LCAD is a homotetramer containing one FAD per 43 kDa subunit with Glu291 as the catalytic base. LCAD substrate specificity overlaps those of VLCAD and MCAD, and in addition includes unsaturated and branched-chain substrates. Here we present the three-dimensional structure of human LCAD, revealing an unusually large substrate-binding cavity not previously reported in eucaryotic ACADs. The structural basis for the unique substrate binding cavity can be seen in the long E helix, where Pro132 is located in a position to cause unwinding of about two turns of the E helix, thus creating a large cavity.

In addition, the structure of the Glu291Gln (E291Q) mutant complexed with lauric acid has been determined to 2.0 Å resolution. Although we obtained crystals of the LCAD E291Q mutant co-crystallized with substrate lauroyl-CoA (C12-CoA), density for the CoA moiety is not observed, and only weak electron density of the alkyl chain portion is observed, likely due to hydrolysis of C12-CoA during the crystallization process. The crystal packing of the LCAD E291Q P1 form is very similar to the crystal packing of the wild type LCAD P21 crystal, except that, in the P1 space group, the adenine ring binding site now has moved slightly away from the symmetry related A and B molecules to avoid steric clashes, transforming the P21 space group of wild type LCAD to the P1 space group of the E291Q mutant crystal. The chain starts at Glu34 in all four monomers of the mutant LCAD structure. The structure of the catalytic residue mutant, E291Q, with the lauroyl moiety of C12-CoA bound in the active site shows that Gln291, extending out from helix G, is located at the active site close to the Cα-Cβ bond of the substrate. In all eight monomers of E291Q LCAD, electron densities for the substrate fatty-acyl portion are weak and interactions with cavity-forming hydrophobic residues are not seen. The LCAD binding cavity is deeper and wider compared to those of other mammalian ACADs, accounting for the lack of specific interactions between the fatty acyl chain of C12-CoA (bound substrate) and cavity-forming residues. Likewise, the overall structure of ligand-bound E291Q LCAD is similar to those of both the ligand bound and unliganded wild-type structures. In all LCAD structures lacking bound CoA derivatives (all eight monomers of mutant LCAD, all four monomers of ligand-free wild type LCAD, and the C and D monomers of the ligand-bound wild type LCAD), residues Ser179 through Gln182 in the vicinity of the CoA moiety of the substrate are relatively disordered in the absence of ligand.

>[8x]GGEERLETPSAKKLTDIGIRRIFSPEHDIFRKSVRKFFQEEVIPHHSEWEKAGEVSREVWEKAGKQGLLGVNIAEHLGGIGGDLYSAAIVWEEQAYSNCSGPGFSIHSGIVMSYITNHGSEEQIKHFIPQMTAGKCIGAIAMTEPGAGSDLQGIKTNAKKDGSDWILNGSKVFISNGSLSDVVIVVAVTNHEAPSPAHGISLFLVENGMKGFIKGRKLHKMGLKAQDTAELFFEDIRLPASALLGEENKGFYYIMKELPQQRLLIADVAISASEFMFEETRNYVKQRKAFGKTVAHLQTVQHKLAELKTHICVTRAFVDNCLQLHEAKRLDSATACMAKYWASELQNSVAYDCVQLHGGWGYMWEYPIAKAYVDARVQPIYGGTNEIMKELIAREIVFDK>GPLGSMSFTNATFSQVLDDLSARFILNLPAEEQSSVERLCFQIEQAHWFYEDFIRAQNDQLPSLGLRVFSAKLFAHCPLLWKWSKVHEEAFDDFLRYKTRIPVRGAIMLDMSMQQCVLVKGWKASSGWGFPKGKIDKDESDVDCAIREVYEETGFDCSSRINPNEFIDMTIRGQNVRLYIIPGISLDTRFESRTRKEISKIEWHNLMDLPTFKKNKPQTMKNKFYMVIPFLAPLKKWIKKRNIAN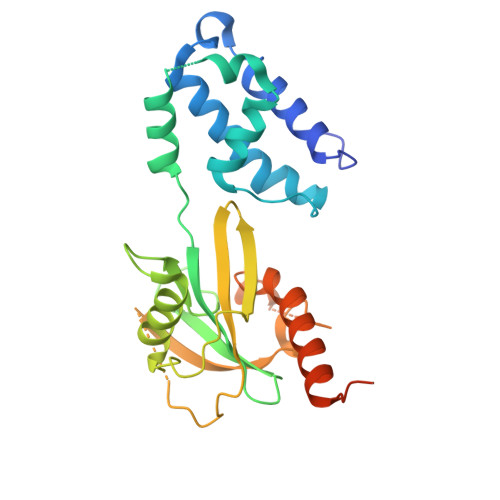NTTKEKNISVDVDADASSQLLSLLKS[2x]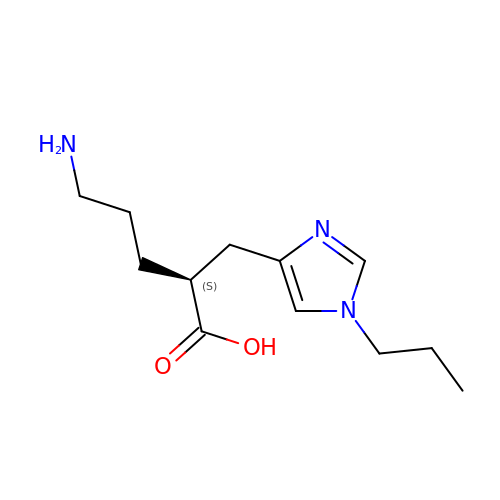(2S)-5-AMINO-2-[(1-PROPYL-1H-IMIDAZOL-4-YL)METHYL]PENTANOIC ACID | C12 H21 N3 O2 | OTDGPKRCQXSTPV-JTQLQIEISA-N>[2x]PPYTVVYFPVRGRCAALRMLLADQGQSWKEEVVTVETWQEGSLKASCLYGQLPKFQDGDLTLYQSNTILRHLGRTLGLYGKDQQEAALVDMVNDGVEDLRCKYISLIVTN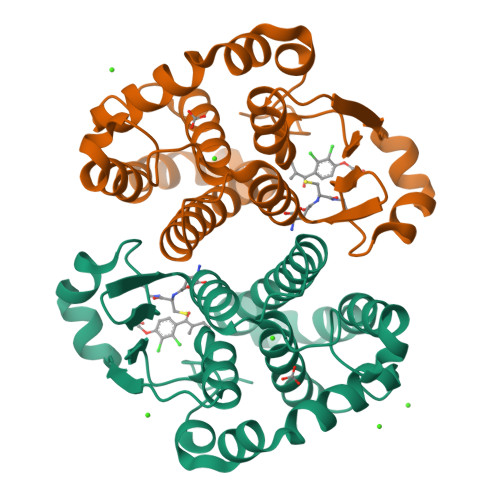YEAGKDDYVKALPGQLKPFETLLSQNQGGKTFIVGDQISFADYNLLDLLLIHEVLAPGCLDAFPLLSAYVGRLSARPKLKAFLASPEYVNLPINGNGKQ>[60x]MEAVLTK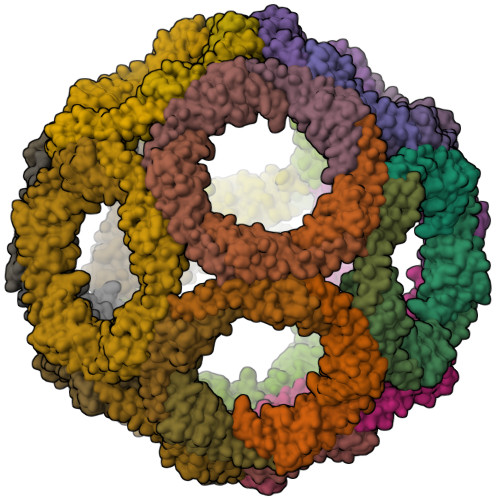LDQEEKKALQNFHRCAWEETKNIINDFLEIPEERCTYKFNSYTKKMELLFTPEFHTAWHEVPECREFILNFLRLISGHRVVLKGPTFVFTKEIKNLGIPSTINVDFQANIENMDDLQKGNLIGKMNIKEG> GPDSMSYRKLKTIPWLELYDILRSHRNPTRSPQRPHDIKVIVDTMLIGFGKNLRRVGIDVILPKDVSDFRKYLKEIERVGGEHLRHIITVPSKSYEALKMDYDNYTIAIPELNNMSPVDQLIEFFDLFNVDIRPEDVYPRCTECNSRLQIKFPGPVLHFLHQYCVIHVQNVYRADMSEFPLEEWWNRMLHINPDDYDGVKVEMSRPSPTSKWIVATVPTGCLHITRQTALHTNLPDGIEVRIHKVPDDEFKRRNLSFYVCGECGTVACDGRG;> GPDSMDEDEIDDEDTYGTRGTSNIPMRPFIKDLAPTMLQLLRQDKTDSEKPQSALCTVVQKIDGFAILYTAKRDVINVLLQERSCEGLERSPQLGDVAFFDILPRRIETKDRLIFKIPYTHIAVKKKPDTPDSLLKIDCFKNSVRCFGGVLEMKVKIALSKPELVVEQYHDNTEMNSDHHFYYLKATNGVLVTIPKERLLNHLNSKLSADFDLIAWVVHRKPIGNVSLHIGKGGEAYQQFTNGDIRELPPL

The MUT-7 family of 3′–5′ exoribonucleases is evolutionarily conserved across the animal kingdom and plays essential roles in small RNA production in the germline. Most MUT-7 homologues carry a C-terminal domain of unknown function named MUT7-C appended to the exoribonuclease domain. Caenorhabditis elegans MUT-7 contains a specific insertion within MUT7-C, which allows binding to MUT-8 and, consequently, MUT-7 recruitment to germ granules. In addition, in C. elegans and human MUT-7, the MUT7-C domain contributes to RNA binding and is thereby crucial for ribonuclease activity.

Further trimming of a few external amino acids on the CTDs of MUT-7 and MUT-8 yielded diffracting crystals with one copy of the complex in the asymmetric unit. Structural analysis using Foldseek revealed that both subdomains show similarity to oligonucleotide/oligosaccharide-binding (OB)-folds flanked by additional secondary structure elements. MUT-8 Asp330, in turn, interacts with MUT-7 Lys838, which is further stabilized by the interaction with MUT-8 Asp328 and Glu551. Next to MUT-7 Arg853, Thr855 forms a hydrogen bond to MUT-8 Arg536. In humans, the insertion is mainly disordered, but in C. elegans (and other Caenorhabditis species), it forms a four-stranded β-sheet (aa 784–868). The surface of the β-sheet participates in MUT-8 binding and mutations in this region (R853E, T855E) abolish complex formation. Interestingly, the zinc finger does not seem to be directly involved in RNA binding but rather in coordinating the CTD-N and the CTD-C parts of the MUT7-C domain. The interaction between MUT-8 and MUT-7 is mediated by the two folded CTDs forming a tight complex. Mutations in the MUT7-C β-sheet prevent MUT-8 binding and result in RNAi resistance.> MEQEHTE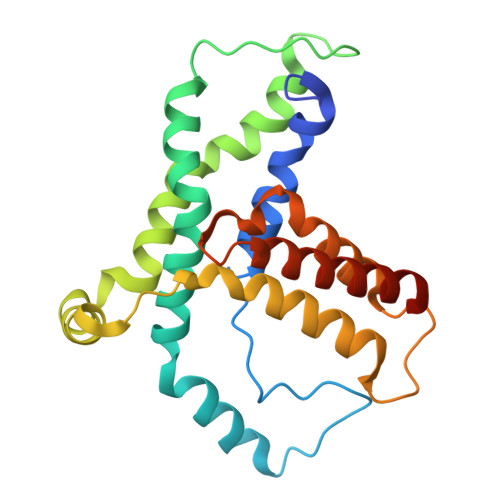ILRGLRFTLLFVQHVLEIAALKGSASEAAGGPEYQLQESVVADQISLLSREWGFAEQLVLYLKVAELLSSGLQSAIDQIRAGKLCLSSTVKQVVRRLNELYKASVVSCQGLSLRLQRFFLDKQRLLDRIHSITAERLIFSHAVQMVQSAALDEMFQHREGCVPRYHKALLLLEGLQHMLSDQADIENVTKCKLCIERRLSALLTGICA>[6x]PIISEGNRNRHRAWALRELQDIKK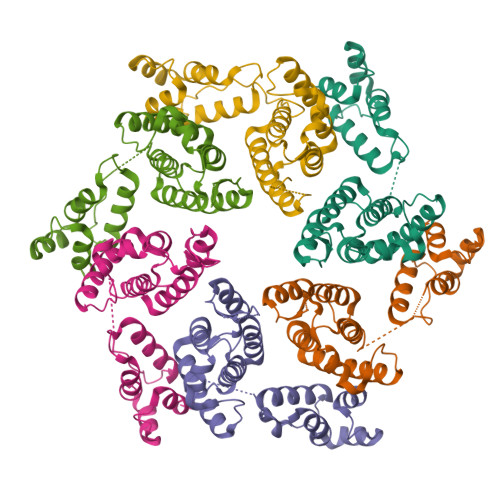EIENKAPGSQVWIQTLRLAILQADPTPADLEQLCQYIASPVDQTAHMTSLTAAIAAAEAANTLQGFNPQNGTLTQQSAQPNAGDLRSQYQNLWLQAWKNLPTRPSVQPWSTIVQGPAESYVEFVNRLQISLADNLPDGVPKEPIIDSLSYANANKECQQILQGRGLVAAPVGQKLQACAHWAPKVKQPAVL>[4x]VKRRADPDPMKNTCKLLVVADHRFYRYMGRGEESTTTNYLIELIDRVDDIYRNTAWDNAGFKGYGIQIEQIRILKSPQEVKP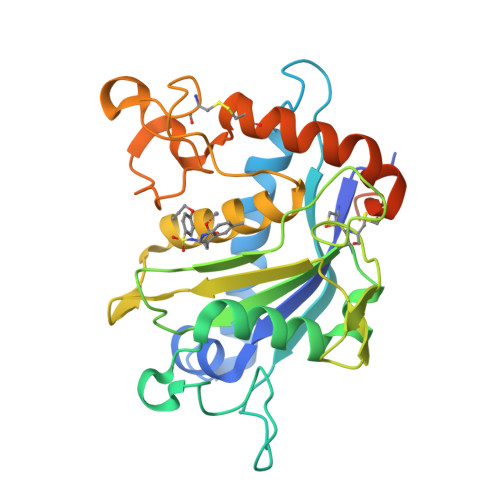GEKHYNMAKSYPNEEKDAWDVKMLLEQFSFDIAEEASKVCLAHLFTYQDFDMGTLGLAYVGSPRANSHGGVCPKAYYSPVGKKNIYLNSGLTSTKNYGKTILTKEADLVTTHELGHNFGAEHDPDGLAECAPNEDQGGKYVMYPIAVSGDHENNKMFSQCSKQSIYKTIESKAQECFQERSNKVCGNSRVDEGEECDPGSHHHHHH>MREYKVVVLGSGGVGKSALTVQFVTGTFIEKYDPTIEDFYRKEIEVDSSPSVLEILDTAGTEQFASMRDLYIKNGQGFILVYSLVNQQSFQDIKPMRDQIIRVKRYEKVPVILVGNKVDLESEREVSSSEGRALAEEWGCPFMETSAKSKTMVDELFAEIVRQMNYA[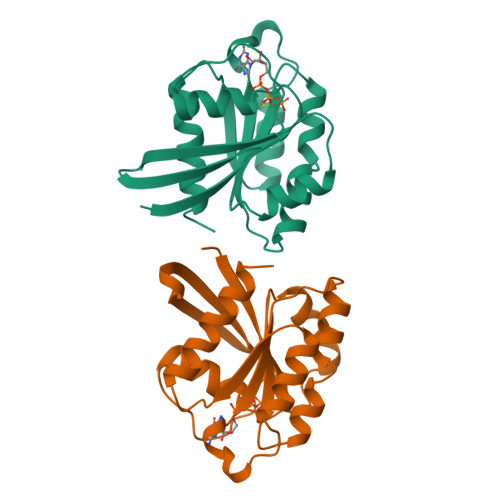2x]>[2x]MTGMSREEVESLIQEVLEVYPEKARKDRNKHLAVNDPAVTQSKKCIISNKKSQPGLMTIRGCAYAGSKGVVWGPIKDMIHISHGPVGCGQYSRAGRRNYYIGTTGVNAFVTMNFTSDFQEKDIVFGGDKKLAKLIDEVETLFPLNKGISVQSECPIGLIGDDIESVSKVKGAELSKTIVPVRCEGFRGVSQSLGHHIANDAVRDWVLGKRDEDTTFASTPYDVAIIGDYNIGGDAWSSRILLEEMGLRCVAQWSGDGSISEIELTPKVKLNLVHCYRSMNYISRHMEEKYGIPWMEYNFFGPTKTIESLRAIAAKFDESIQKKCEEVIAKYKPEWEAVVAKYRPRLEGKRVMLYIGGLRPRHVIGAYEDLGMEVVGTGYEFAHNDDYDRTMKEMGDSTLLYDDVTGYEFEE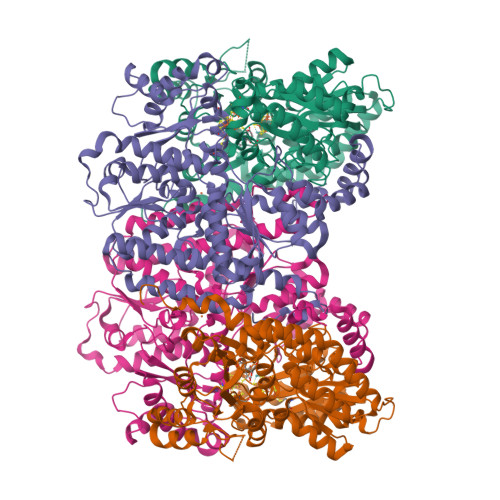FVKRIKPDLIGSGIKEKFIFQKMGIPFREMHSWDYSGPYHGFDGFAIFARDMDMTLNNPCWKKLQAPWEASEGAEKVAASA;>MSQQVDKIKASYPLFLDQDYKDMLAKKRDGFEEKYPQDKIDEVFQWTTTKEYQELNFQREALTVNPAKACQPLGAVLCALGFEKTMPYVHGSQGCVAYFRSYFNRHFREPVSCVSDSMTEDAAVFGGQQNMKDGLQNCKATYKPDMIAVSTTCMAEVIGDDLNAFINNSKKEGFIPDEFPVPFAHTPAFVGSHVTGWDNMFEGIARYFTLKSMDDKVVGSNKKINIVPGFETYLGNFRVIKRMLSEMGVGYSLLSDPEEVLDTPADGQFRMYAGGTTQEEMKDAPNALNTVLLQPWHLEKTKKFVEGTWKHEVPKLNIPMGLDWTDEFLMKVSEISGQPIPASLTKERGRLVDMMTDSHTWLHGKRFALWGDPDFVMGLVKFLLELGCEPVHILCHNGNKRWKKAVDAILAASPYGKNATVYIGKDLWHLRSLVFTDKPDFMIGNSYGKFIQRDTLHKGKEFEVPLIRIGFPIFDRHHLHRSTTLGYEGAMQILTTLVNSILERLDEETRGMQATDYNHDLVR[2x]>MRTMPDAPALHLTAIDSHAHVFSRGLNLASQRRYAPNYDAPLGDYLGQLRAHGFSHGVLVQPSFLGTDNRYLLSALQTVPGQLRGVVMLERDVEQATLAEMARLGV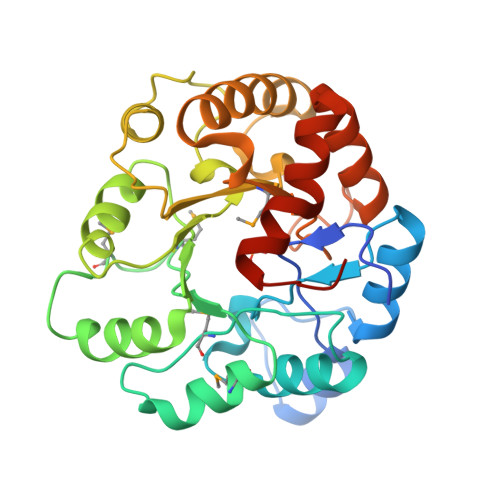RGVRLNLMGQDMPDLTGAQWRPLLERIGEQGWHVELHRQVADIPVLVRALQPYGLDIVIDHFGRPDARRGLGQPGFAELLTLSGRGKVWVKVSGIYRLQGSPEENLAFARQALCALEAHYGAERLMWGSDWPHTQHESEVSFGSAVEQFEALGCSAQLRQALLLDTARALFGFELEHHHHHH[2x]>TQKPSLYRVLILNDDYTPAEFVVYVLERFFNKSREDATRIMLHVHQNGVGVCGVYTYEVAETKVAQVIDSARRHQHPLQCTMEKD[2x];> L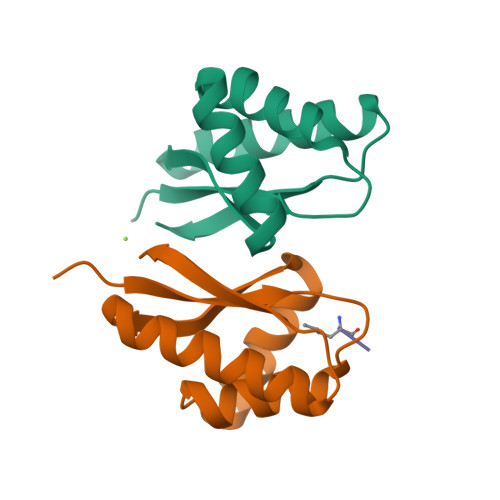LFVQRDSKE> MGNDDIRQVYYRDKGISHAKAGRYSEAVVMLEQVYDADA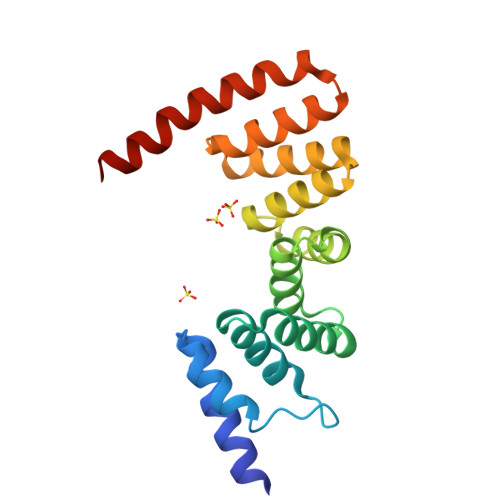FDVEVALHLGIAYVKTGAVDRGTELLERSIADAPDNIKVATVLGLTYVQVQKYDLAVPLLVKVAEANPVNFNVRFRLGVALDNLGRFDEAIDSFKIALGLRPNEGKVHRAIAYSYEQMGSHEEALPHFKKANELDERSAVELALVPR6-fluoro-2-(2'-fluoro[1,1'-biphenyl]-4-yl)-N-methoxy-3-methylquinoline-4-carboxamide 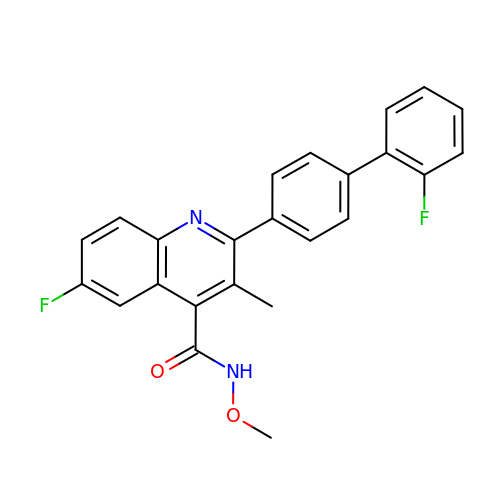| C24 H18 F2 N2 O2 | XPBXJYBHOVBFDA-UHFFFAOYSA-N>GAGEARLEEAVNRWVLKFYFHEALRAFRGSRYGDFRQIRDIMQALLVRPLGKEHTVSRLLRVMQCLSRIEEGENLDCSFDMEAELTPLESAINVLEMIKTEFTLTEAVVESSRKLVKEAAVIICIKNKEFEKASKILKKHMSKDPTTQKLRNDLLNIIREKNLAHPVIQNFSYETFQQKMLRFLESHLDDAEPYLLTMAKKALK[2x];>SQETFEEKYRLSPTLSSTKGH[2x]

MCPH1 plays important roles in DDR upon induction of double-strand breaks (DSBs). It contains two BRCA1 C-terminus (BRCT) domains at its C-terminus that mediate its interaction with the DNA damage marker γ-H2AX. The shelterin components TRF1 and the TRF2-RAP1 heterodimer specifically recognize double stranded telomeric repeats, while POT1 binds the single stranded (ss) 3’ overhang. A previous report showed that MCPH1 interacts with the TRF Homology (TRFH) domain of TRF2 and localizes at dysfunctional telomeres.

Analysis of the human MCPH1 amino acid sequence revealed the presence of a 330YRLSP334 sequence typical of the TRFH-binding motif (TBM) Y/F/H-X-L-X-P (where X is any amino acid) found in proteins that interact with TRF2, including Apollo/hSNM1B, PNUTS, SLX4, and NBS142–45. To understand the structural basis of this interaction, we solved the crystal structure of TRF2TRFH–MCPH1TBM complex at a resolution of 2.15 Å by molecular replacement. As predicted, the binding mode of MCPH1TBM to TRF2TRFH closely resembles the interaction between ApolloTBM and TRF2TRFH 43. MCPH1TBM binds to TRF2TRFH in an extended conformation with a short helix at the N-terminus across the concave face of each TRF2 subunit, and involves an extensive set of interactions, including both Van der Waals contacts and electrostatic polar interactions. The most critical interaction interface is the central portion of MCPH1TBM (330YRLSP334). MCPH1Y330 fits into a hydrophobic cleft formed by the aliphatic side chain of TRF2L101 and TRF2R102, and the hydroxyl group of MCPH1Y330 forms two hydrogen bonds with TRF2S98 and TRF2E94. MCPH1L332 is completely buried in a deep pocket surrounded by hydrophobic residues from α2 and α3 of TRF2, and MCPH1P334 stacks with the aromatic ring of TRF2F120. The backbone carbonyl of MCPH1R331 forms a hydrogen bond with TRF2R109. Isothermal titration calorimetry (ITC) confirmed the MCPH1TBM–TRF2TRFH interaction with an equilibrium dissociation constant (KD) of 0.24 μM. Mutating any one of the three conserved residues in the TRFH-interacting motif (Y330, L332, or P334) either completely abolished this interaction or greatly reduced it, confirming the importance of these hydrophobic contacts in  mediating the MCPH1TBM–TRF2TRFH interaction.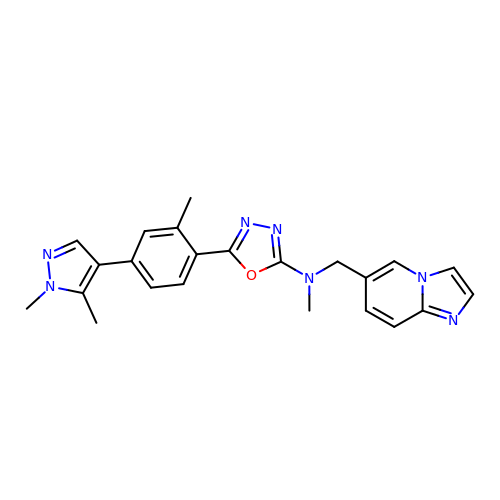5-[4-(1,5-dimethylpyrazol-4-yl)-2-methyl-phenyl]-~{N}-(imidazo[1,2-a]pyridin-6-ylmethyl)-~{N}-methyl-1,3,4-oxadiazol-2-amine | C23 H23 N7 O | SERBYZUNBVTZJZ-UHFFFAOYSA-N Pro-survival homologs (six in humans: Bcl-2, Bcl-xL, Bcl-w, Mcl-1, Bfl-1 and Bcl-B) are structurally similar, but oppose apoptosis by binding and inhibiting Bak and Bax, as well as sequestering pro-apoptotic BH3-only proteins (BOPs). Interactions between BCL2 members are mediated by an amphipathic, helical BH3 motif that recognizes a conserved hydrophobic cleft present in the effectors and pro-survival proteins. Here we describe the computational design and experimental characterization of specific, high affinity protein inhibitors for all six pro-survival BCL2 homologs. As confirmed by biochemical analyses and X-ray crystal structures, the designed proteins engage the BH3-binding grooves of their specific target pro-survival BCL2 family members.

Thus, in lieu of generating a combinatorial library, single amino acid mutants were screened with BLI, and three mutations improving both specificity and affinity were combined in αBCL2. For example, the binding mode of αBCL2 in the hydrophobic cleft of Bcl-2 differs significantly between the crystal structure and backbone-constrained design model; after Bcl-2 alignment, Cα backbones of the αBCL2 crystal and design models deviate by 4.0 Å RMSD (average amongst the two complexes observed in the asymmetric unit). The SSM-guided mutation of 2-CDP06 core residue G107R is likely responsible, requiring the first and third helices of αBCL2 to shift relative to the BH3-mimetic helix and positioning the third helix much further from Bcl-2 than the αMCL1•Mcl-1 binding mode. The αBCL2 binding mode enables electrostatic interactions between αBCL2 R107 and Bcl-2 residues D111 and E114. SSM-guided αBCL2 mutation G107R contributes additional polar contacts with Bcl-2. (B) Designed αBCL2 residue R50 is tolerated by a more spacious Bcl-2 binding pocket and interacts with Bcl-2 E114. Designed αBCL2 residue D47 is partially satisfied by Bcl-2 R129. The αBCL2•Bcl-2 crystal structure reveals that Bcl-2 residue D111 makes a hydrogen bond with αBCL2 N57, satisfying a polar atom that is likely buried in the interface when binding other homologs. Like αMCL1, αBCL2 expands the classic BH3 interface by 452 Å2.

>MAHAGRTGYDNREIVMKYIHYKLSQRGYEWDAGDVGAAPPGAAPAPGIFSSQPGHTPHPAASRDPVARTSPLQTPAAPGAAAGPALSPVPPVVHLTLRQAGDDFSRRYRRDFAEMSSQLHLTPFTARGRFATVVEELFRDGVNWGRIVAFFEFGGVMCVESVNREMSPLVDNIALWMTEYLNRHLHTWIQDNGGWDAFVELYGPSMRLEHHHHHH[2x];>MADPKKVLDKAKDEAENRVRELKQRLEELYKEARKLDLTQEMRQELVDKARAASLQANGDIFYAILRALAEAEKLKKAGLVNSQQLDELKRRLEELAEEARRKAEKLRDEFRLKLEYG[2x]>[2x]SMNYFVGNSLGVNLTGIEKAIINRLNLFKEMGRPAQCVFLSWNRYLYRNAQNYITSSDYINMYDFFQEATYLERNEPFDWLSYWTDECHYTLKHVENSHDFRIYDQERFLMYAHFQDPKYRILDYVNHFDSQRRKVKRDFYDVRGFLSCSRILVDKQQTLCEFFYNPEGDTKLEKYFSYKDGKPE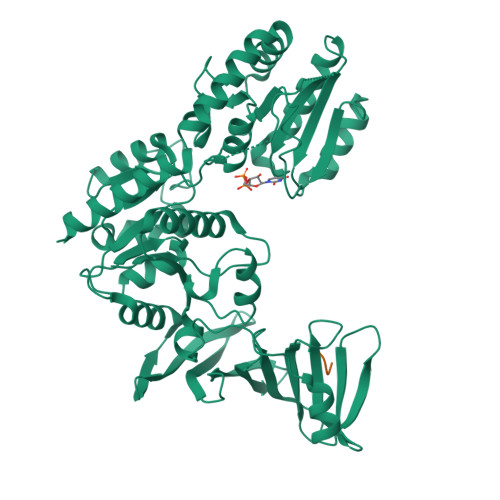VQKIIVYYANKQYFFNNETELGAFFIKQLYQHGDLFFSDRNVYTAPIFNLTPESIPVVAVLHSTHIKNIDALDSSPFKNVYKAMFENLSRYRAIIVSTEQQKLDVEKRINHTIPVVNIPVGYSETIDTPVQTLDQRSVKLISVARYSPEKQLHQQIELIKRLVSYVPKIELHMYGFGSESKKLNELIQKYGLENHVYLRGFLSNLDQEYSDAYLSLITSNMEGFSLALLESLAHGVPVISYDIKYGPNELITSDFNGYLITKNDEDALFDKVKYVIDHPEVQQRLSKGSLAKAQQYSKASLIKQWDQFVRLILEHHHHHH;>DSDSD[2x]> NVNLEQLKQKAESGEAKAQLELGYRYFQGNETTKDLTQAMDWFRRAAEQGYTPAEYVLGLRYMNGEGVPQDYAQAVIWYKKAALKGLPQAQQNLGVMYHEGNGVKVDKAESVKWFRLAAEQGRDSGQQSMGDAYFEGDGVTRDYVMAREWYSKAAEQGNVWSCNQLGYMYSRGLGVERNDAISAQWYRKSATSGDELGQLHLADMYYFGIGVTQDYTQSRVLFSQSAEQGNSIAQFRLGYILEQGLAGAKEPLKALEWYRKSAEQGNSDGQYYLAHLYDKGAEGVAKNREQAISWYTKSAEQGDAT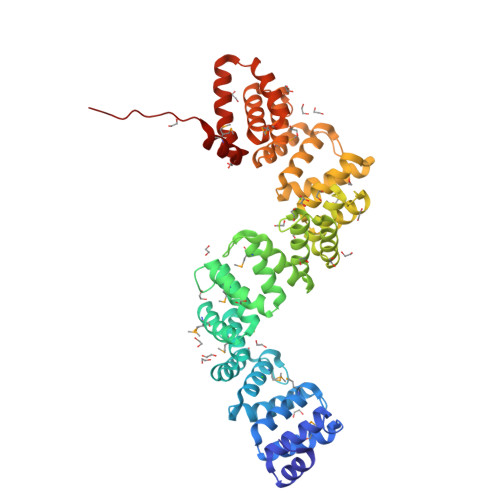AQANLGAIYFRLGSEEEHKKAVEWFRKAAAKGEKAAQFNLGNALLQGKGVKKDEQQAAIWMRKAAEQGLSAAQVQLGEIYYYGLGVERDYVQAWAWFDTASTNDMNLFGTENRNITEKKLTAKQLQQAELLSQQYIEKYAPEAWARMQKLKAQSAVKTGNK> GPAASAGRIER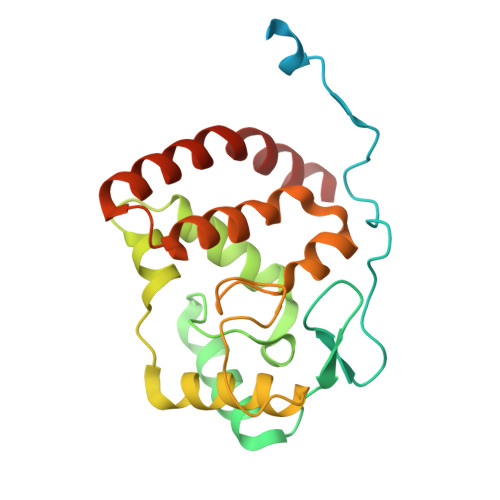RRARAAVAGRDATGRFTAGQPRRVELDADATSGAFYARYRDGYVSGEPWPGAGPPPPGRVLYGGLGDSRPGLWGAPEAEEARRRFEASGAPAAVWAPELGDAAQQYALITRLLYTPDAEAMGWLQNPRVVPGDVALDQACFRISGAARNSSSFITGSVARAVPHLGYAMAAGRFGWGLAHAAAAVAMSRRYDRAQKGFLLTSLRRAYAPLLARENAALTG>[4x]MRVLVTGGAGFIGSHIVEDLLARGLEVAVLDNLATGKRENVPKGVPFFRVDLRDKEGVERAFREFRPTHVSHQAAQASVKVSVEDPVLDFEVNLLGGLNLLEACRQYGVEKLVFASTGGAIYGEVPEGERA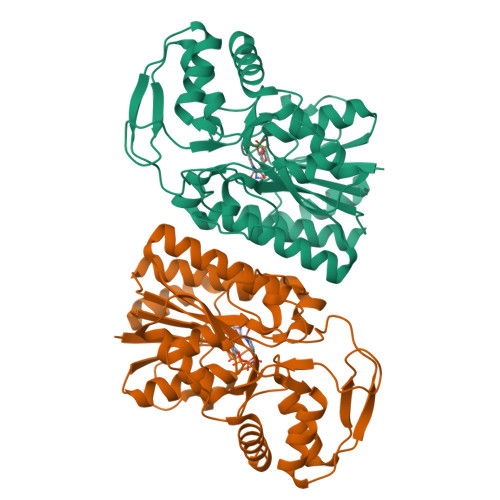EETWPPRPKSPYAASKAAFEHYLSVYGQSYGLKWVSLRYGNVYGPRQDPHGEAGVVAIFAERVLKGLPVTLYARKTPGDEGCVRDYVYVGDVAEAHALALFSLEGIYNVGTGEGHTTREVLMAVAEAAGKAPEVQPAPPRPGDLERSVLSPLKLMAHGWRPKVGFQEGIRLTVDHFRGAV>[2x]MSAHRTLLLRLSDSGEPVTSCSYGQGVLTLPSLPLPQGKKLGDMPVYTVKLAIPAGSPVTRDGLIWTNCPPDFSTQFDREKFYKKIIKTSFHEDDHIDLDIYVPGTYCFYLSFKNDKDELETTRKFYFVVLPILSVNDKFIPLNSIAMQSVVSKWMGPTIKDWEKVFARVASKKYNMIHFTPLQHRGESNSPYSIYDQLEFDPTVFKSEKEVADMVERLRTEHNILSLTDIVFNHTANNSQWLLDHPEAGYNHKTSPHLISAIELDKKLLDFSEQMEALGYPVDLKTVDDLIKVMDGIKEHVIGELKLWEFYVVDVKQTVSELREKWGNSKSWSDDNIPSKDDSTNLAQFVRDNATEPGFGSLGERGSNKINIDKFAAILKKLHSEDYNNGIEELATKILNDINLPFYKEYDDDINEVLEQLFNRIKYLRIDDHGPKQGPITKKLPLSEPYFTRFKAKDGEEYALANNGAIWDGNPLVDFASSQSKAYLRREVIVWGDCVKLRYGKGPSDSPYLWERMSKYVEMNARIFNGFRIDNCHSTPLHVGQYFLDVARRVNPNLYVVAELFSGSEAMDCLFVERLGISSLIREAMQAWSEEELSRLVHRHGGRPIGSYKFVPLDDFPYPADVKIDEEYCAYNPDDHSVKCVSEIMIPKTLTATPPHALFMDCTHDNETPNQKRTVEDTLPNAALVAFCSSAIGSVYGYDEVFPQLLDLVQEKRTYSCAENTGISKVKTLLNNMREEIASEAVDIEDSEMHVHHDGQYITFHRTNAKNGKGWYLVARTKFHSSGDQMLPRIKLSQTKATFKAAFSLERTGDAPISDEIIEGIPTKLRELTGFDIGF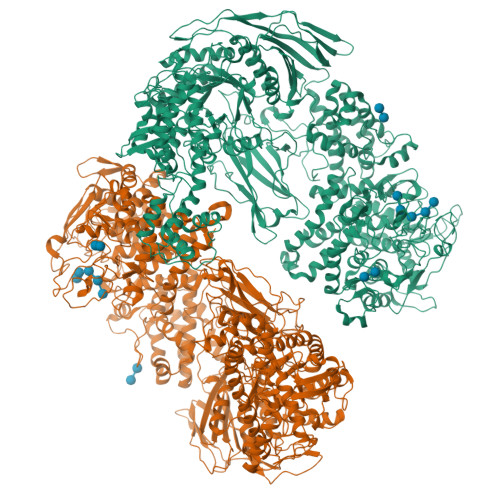DENTKETSILLPQDFPQGSIVIFETQQLGIDDSLDHFIRSGAIKATEKLSLESINYVLYRAEQEEYDYSEGRSGAYDIPDYGKPVYCGLQGWVSILRKIIFYNDLAHPLSNNLRNGHWAVDYVVNRLDLYKDKEGVAEVQEWLRSRMERIKQLPSYLVPSFFALVVGIMYGCCRLRAMQLMSDNVGKSTVFVQSLAMTSIQMVSAMKSTSILPDQNIAAMAAGLPHFSTNYMRCWGRDVFISLRGLLLTTGRYEEAKEHILAFAKTLKHGLIPNLLDAGRNPRYNARDAAWFFVQAIQDYVTIVPGGVSLLQEKVTRRFPLDDEYIPYDDPKAFSYSSTIEEIIYEILNRHAGGIKYREANAGPNLDRVMKDEGFNVEVNVDWETGLIHGGSQFNCGTWMDKMGESEKANSVGVPGTPRDGAAVEINGLLKSCLRFVLQLSKDGKFKYTEVTKPDGSKISLSSWNDLLQENFERCFYVPKNKEDDNKFEIDATIINRRGIYKDLYRSGKPYEDYQFRPNFTIAMVVAPELFTPDYAAGAIELADQVLRGPVGMRTLDPSDYNYRPYYNNGEDSDDFATSKGRNYHQGPEWVWCYGYFIRAYHYFNFLTNPKCQVEGSAKKLKPSSYLYRKLYSRLLKHREWIENSPWAGLAELTNKDGEVCNDSSPTQAWSTGCLLDLFYDLWISYEELEHHHHHH> MKRYPGLIGLLVVLVSVAGCRFYGYPGGVALTLAQIEAASEQVAQD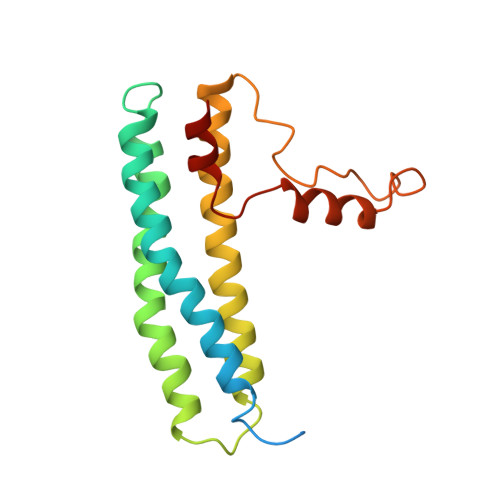LEQALAELEALRLLARRDETLAPYVAQYEAILEAHQQAVLEFEHWKEQVAAHPGDYRRANRTLGAITARHEALLQQYADVAWAVAQHVNPALLARAYTSSGPRFFFYVVPPQYARQVNEQAVPPLQVVRYLAAQLS>[2x]MKVKGLSVLVVCTGNLCRSPMAEIILRDKIRQKRLNIQVRSAGTLKTGKTMPDDKALQALQDYGYHPMVNPVQQV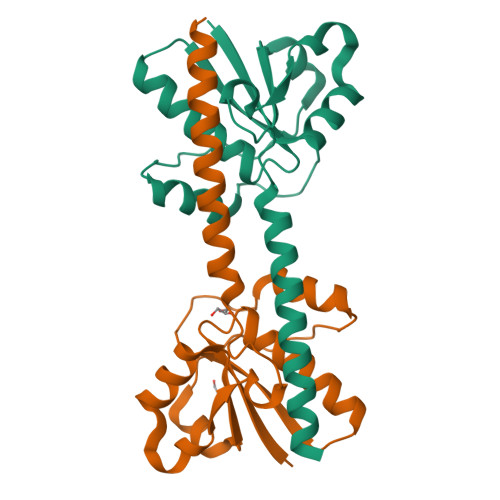TQQDFIEHDFIYAMDRTNLADLLDICPAEHKNKLALFLSKANRQEKEVPDPYRRSSEFFQRTALLIESGAVALVDSWQEQGINACNENLSQ8-aminooctanoic acid | C8 H17 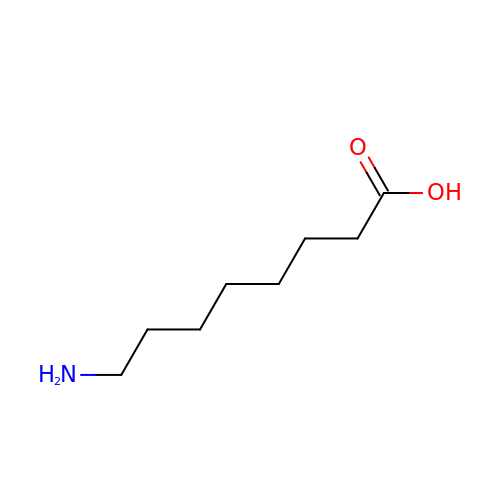N O2 | UQXNEWQGGVUVQA-UHFFFAOYSA-N> MQRREFLKLSALGVGAMALRGSGPAKALKAPWYAQEVKSVYQI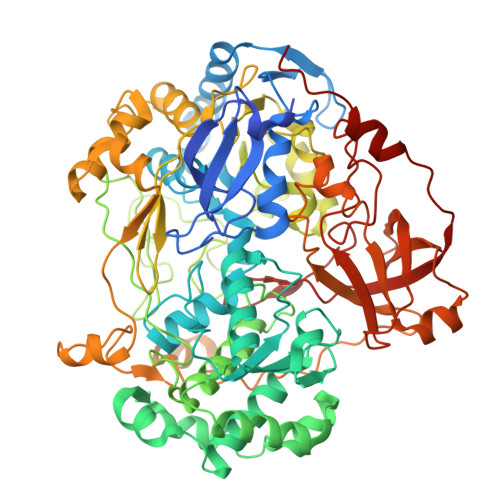CEGCFWRCGIVAHAVGNRVYKVEGYEANPKSRGRLCPRGQGAPQTTYDPDRLKRPLIRVEGSQRGEGKYRVATWEEALDHIAKKMLEIREKYGPEAIAFFGHGTGDYWFVDFLPAAWGSPNAAKPSVSLCTAPREVASQWVFGRPIGGHEPIDWENARYIVLIGHHIGEDTHNTQLQDFALALKNGAKVVVVDPRFSTAAAKAHRWLPIKPGTDTALLLAWIHVLIYEDLYDKEYVAKYTVGFEELKAHVKDFTPEWAEKHTEIPAQVIREVAREMAAHKPRAVLPPTRHNVWYGDDTYRVMALLYVNVLLGNYGRPGGFYIAQSPYLEKYPLPPLPLEPAAGGCSGPSGGDHEPEGFKPRADKGKFFARSTAIQELIEPMITGEPYPIKGLFAYGINLFHSIPNVPRTKEALKNLDLYVAIDVLPQEHVMWADVILPEATYLERYDDFVLVAHKTPFIQLRTPAHEPLFDTKPGWWIARELGLRLGLEQYFPWKTIEEYLETRLQSLGLDLETMKGMGTLVQRGKPWLEDWEKEGRLPFGTASGKIELYCQRFKEAGHQPLPVFTPPEEPPEGFYRLLYGRSPVHTFARTQNNWVLMEMDPENEVWIHKEEAKRLGLKEGDYVMLVNQDGVKEGPVRVKPTARIRKDCVYIVHGFGHKAPLMRLAHGRGASDNYLQTRYKLDPISGGAGLRVNFVRLEKAERPRLPSLTGLAKRPFDERRM The mitochondrial ATP synthase is a membrane protein complex that generates most of the ATP in eukaryotic cells. The translocation of protons through the membrane-bound Fo part, mediated by subunit a, drives the rotation of a membrane-embedded c-ring and the attached central stalk, which together form the rotor. The torque of the rotor against the stator subunits induces conformational changes in the (αβ)3 headpiece, thereby triggering catalysis. To reveal how the mitochondrial ATP synthase is modulated by lipids and organised into a dimer shaping discoid cristae in Euglenozoan mitochondria, we determined the structure of the ATP synthase dimer from E. gracilis.

Symmetry expansion of the pseudo-C2-symmetric dimer particles was used to classify individual F1/c-ring monomers into rotational states 1, 2 and 3 (named according to bovine nomenclature; Zhou et al., 2015) and resolve structures at 3.0- to 3.9 Å resolution. Using masked refinement, maps of the membrane region, the rotor and the peripheral stalk tip were refined to 2.8 and 3.3 and 3.8 Å resolution, respectively, enabling the construction of atomic models (Figure 1—figure supplements 1–2). By contrast, subunit b is significantly shorter in E. gracilis, extending only ~65 Å into the matrix, and does not interact with OSCP. This is compensated by extensions of OSCP and subunit d mediating the attachment of the peripheral stalk, which is augmented by two species-specific soluble subunits ATPTB3 and ATPTB4. The additional elements significantly increase the size of the peripheral stalk compared to yeast. The C-terminal OSCP extension contains a 13-residue proline-rich region, followed by 26 residues arranged in two helices (D240-L246, V250-A265), which contact the large matrix extension of subunit d. This interaction is further clamped by ATPTB3 and ATPTB4 of the peripheral stalk tip and p18 on F1. Thus, the E. gracilis peripheral stalk displays a different mode of interaction with the OSCP compared to all other reported ATP synthase structures. ATPTB3 is an isocitrate dehydrogenase ortholog that adopts a Rossman fold located at the tip of the peripheral stalk. The OSCP N-terminal domain contains a structurally conserved bundle of four α-helices, followed by the N-terminal extension with a terminal helix. The N-terminal helix of OSCP connects to the central stalk through an interaction with the C-terminal extension of subunit γ of the central stalk.

> MTAVVKNLAKLPAATSQILTNVSKLQTFHGLLEERRDKYAPLAYHTYDNLKQKTTWHPIAHAWVDEGLPVSKKEYNEYCWLKKDMQRLLPLASPFVFGIYGILPLAVWLSNDGYLPSAFSSKKDIVSKKLEWYSSYGDDLRQQVGPMLQHRLKRHLRGTLNNEHRLMLDEVTESYKEIFYSHYTGQLRDVRKCAHLRLYDGTSTVLLLTNKEPVELTSELLQKWNAIKAAKLSPEEEKKARNEALIEAYKEQELHGGPHVKHMQGYGIPSDTPLLGENAKGDQYTQPPESASIPLEQLEWTGDTVFIPAEYRTEVEDWGRELTKLANQFLLLPWRFVSNAWNQRRLVSWFEEILQEDALIAKEGGVQALSDDELKVALLDRAVIRCDEELTRGDMEARYKEISWLMSLRNPFIVLAWQTGYYRSTYSPEDDLPEASILPKLNRTVLDVDVHNELAPDHPEKPLPRVHPALYPNSHLALAKEVAVLAK;> MAAKTIPFVASTALGERLFAGVQKVLAAAKAPVSLVQTDAKFAPADAKYLLAEPLSAAATGELANKYGLSSKVTSGAASQFYPNSIYPSLNVEVVQNLYALSNPAFSSLSATTTKAVTVKDESAIKLAELQKETERNISSFFRDEANKSVQATLRLACDKAIKTKADKKTVMVVTKPHGDAFDDLLAQVTKSESDGRADELRNSSVSVEPTLVGNAWPKLVMFPEGVNVVVCGPNASGDQVAQLFVGIAGGTGMVAQQLVGDAVVFTSANAEDNENPTGALLAASNLLTALGHEAEAKKIAAAVAKAYTTDRILPKELPGGKADLEAFIDAVAKHASA;> MFRGFRPVLAADAVKFQTLYNVLTGKQHLKDQVPVKDCNLTAIFGASWKADLNKWFDSEYAPKLPAAERDSAKKSLDLYLKRVDLTRYTREELTTYGILACGPGKVDALTEKHLLETGKARLEELTAGLGNKDEGVNAFRKEVEQEGKYANWPAEKSKALADKVIAASP;> MMRRACRIIRPSHVRGVSGVAPTIYLRSKAALPATSTTDVRPQLYALQRFAKAQLKTATEAERAAIEADIARYQEYLDSDLEKLKQDVAEDTAKKQKLIPLLDRYPDVPIEKIPEHANVLLKKIDACLEILSKDIGEVTDAEAHEMYFETSKFQILHIYTGCVASFPEGDVPPGAVECLPGQVIRTKVNGEDVMLEIDEVDPGYQVCWFKPDVPLPENAEILWSYPYEPTAALPTGTTWEEGQANVLIPAEPTPEAAVWPPTPVTNVYAPMAEKLALKSNPELKVLFKEALLQPAKLLPLDVDYQCSHDREVVEAKRDRYLTALVEAEQAPPLPFTPDVLQLQLEHNVLKGELIDRLRALEYTIVTEQLQARLHERRLRGDVIDEWEELDYHPLVRDDTYLAIDFGDPTFGRYIWKLFPHTDGDEECMFKDTRLDVLPPQVNPLNAILAQHTAQTPVHRSLEKRLWTEVRATAVSE;> MHMRRAVSVFGRCRSLNGLRNYAVPSPKYIEIYQSDFSRNAYPLELLGGSHVDFAKLLYSFADQVENKKFEVYVEDFKKLDSIIAEKGPFWAEEKIFQSPTFQGLSEGFKFILGWIQSEGAIDRLENVRLAYKELVNEARKETTATVIVAKEPSGNDLAEIRKQVEELHKESPLKDYKLVLETKVDPSIGGGYILEVCNQVVNRSAAAAAAETAALAKASAAQVDWTSLPAAPPRPSPSAPDTLIRLLGSVVDDLADADKVEQKYGA;> MPSTSPADKDVPMSILHTHGLSYVNWCMSLAPGLLVFEGFFRARYYRSRVPPSRTVLMNGLKMRMFSLARQQAPKIVHKPVLSPIPEHLRLVKNVAQVQIDMLKLLNAQAAK;> LIPVSLVDLININIIFYILLLYTLLLFFIPLFLASINYTYHYIYKYYNYNYNFINNNT> RAVPGGSSPAWTQCQQLSQKLCTLAWSAHPLVGHMDLREEGDEETTNDVPHIQCGDGCDPQGLRDNSQFCLQRIHQGLIFYEKLLGSDIFTGEPSLLPDSPVGQLHASLLGLSQLLQPEGHHWETQQIPSLSPSQPWQRLLLRFKILRSLQAFVAVAAR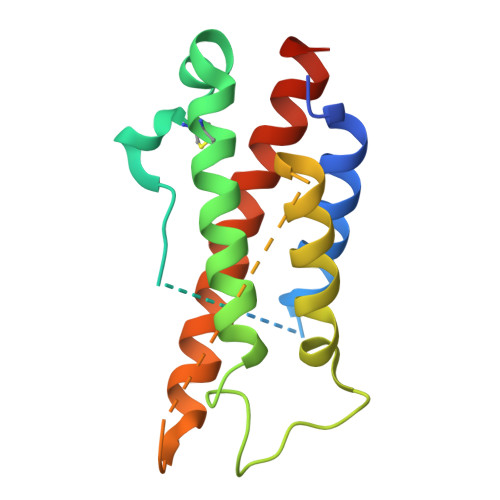VFAHGAATLSPHHHHHH>SNAMLQFSFVSNDVVMTYDGDSGEQIIWVWESLNKFQTVCISRIFNFQLQDLRNPPSTVQDFNDYEYSFNFGTLNNEYITVPGRILSINRDVLIHKSIKLERKVFASERNVSIFGRLSKLLDHTNPIIIGGDKPEAIPKSVFQELQSKFPNTGELDRYANARVHAILAGYLDGMKDARERYEHYLNRKTVIRKTDKLDLEVLNKLEIEKYTLIRDIIQDALNNKTNLSEDDWQSLMIPFITLLFPKYIKVLEKVKIFDYYSNPSAKTNRFIDIALVDANGNLDIIEVKKPFDDKILRKTPYRDNYIPTSELSGGIMQAEKYIFHLSKWGVKGEKELTNAYKNSLPAGMCIRISNPKAII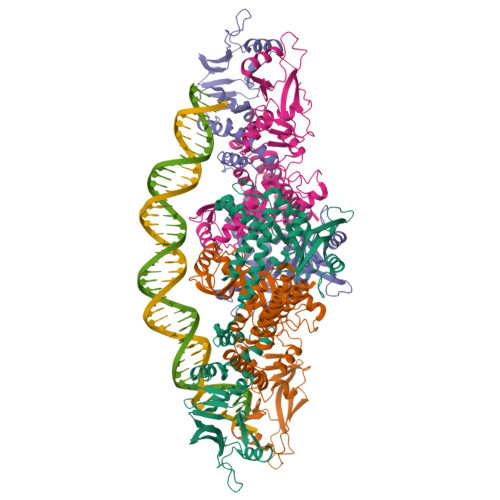IVGRDQIANGNMTDGQLLDFEIIKRKYANMIDILTYDDLLRRLNNTIEALKG[4x]> MAEEWYFGKITRRESERLLLNPENPRGTFLVRESETTKGA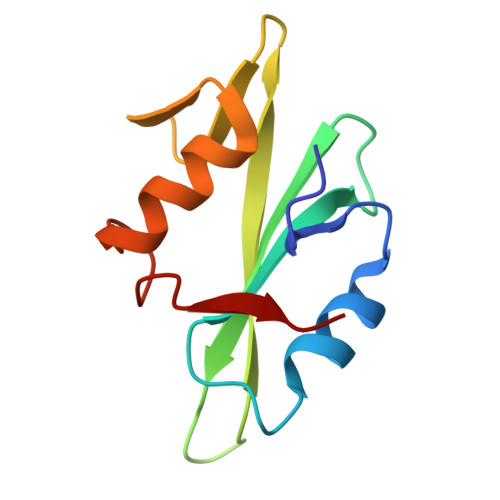YCLSVSDFDNAKGLNVKHYKIRKLDSGGFYIWSRTQFSSLQQLVAYYSKHADGLCHRLTNVCPT>[4x]ARPCIPKSFGYSSVVCVCNATYCDSFDPPTFPALGTFSRYESTRSGRRMELSMGPIQANHTGTGLLLTLQPEQKFQKVKGFGGAMTDAAALNILALSPPAQNLLLKSYFSEEGIGYNIIRVPMASCDFSIRTYTYADTPDDFQLHNFSLPEEDTKLKIPLIHRALQLAQRPVSLLASPWTSPTWLKTNGAVNGKGSLKGQPGDIYHQTWARYFVKFLDAYAEHKLQFWAVTAENEPSAGL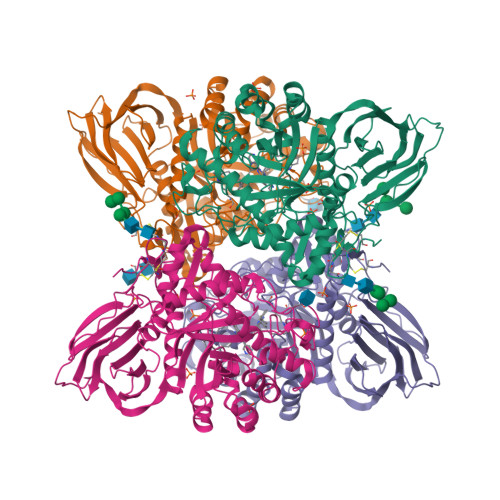LSGYPFQCLGFTPEHQRDFIARDLGPTLANSTHHNVRLLMLDDQRLLLPHWAKVVLTDPEAAKYVHGIAVHWYLDFLAPAKATLGETHRLFPNTMLFASEACVGSKFWEQSVRLGSWDRGMQYSHSIITNLLYHVVGWTDWNLALNPEGGPNWVRNFVDSPIIVDITKDTFYKQPMFYHLGHFSKFIPEGSQRVGLVASQKNDLDAVALMHPDGSAVVVVLNRSSKDVPLTIKDPAVGFLETISPGYSIHTYLWRRQ> GG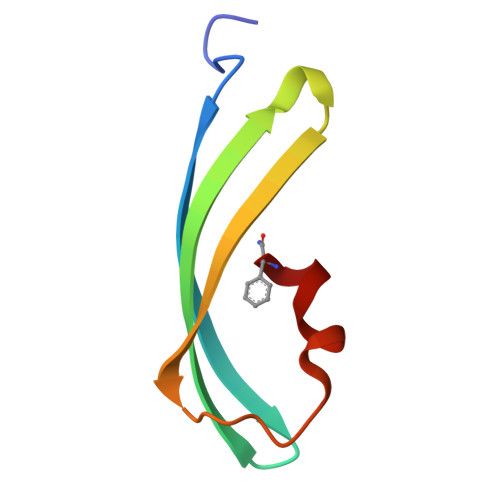AIKPDMKINLRMEGNVNGHHFVIDGDGTGKPFEGKQSMDLEVKEGGPLPFAFDILTTAF> SLWQFGKMINYVMGESGVLQYLSYGCYCGLGGQGQPTDATDRCCFVHDCCYGKVTGCNPKIDSYTYSKKNGDVVCGG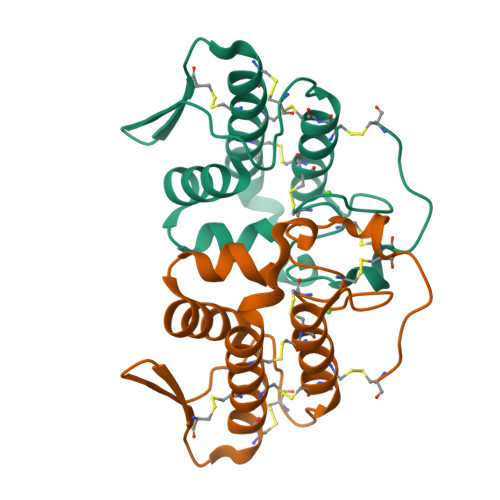DNPCKKQICECDRVATTCFRDNKDTYDIKYWFYGAKNCQEKSEPC4-[1-(4-hydroxyphenyl)ethyl]phenol | C14 H14 O2 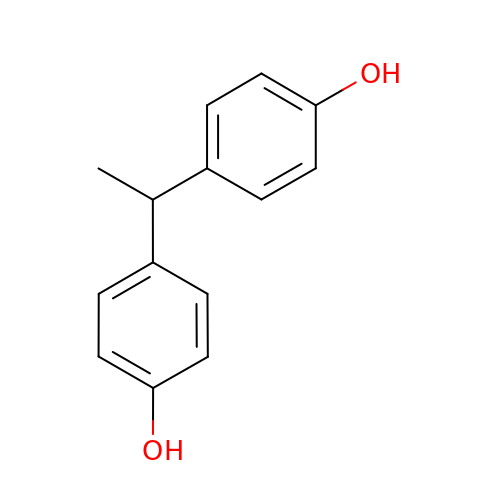| HCNHNBLSNVSJTJ-UHFFFAOYSA-N> MDLMPLEKARAIEIAFDNVFHNTKIPD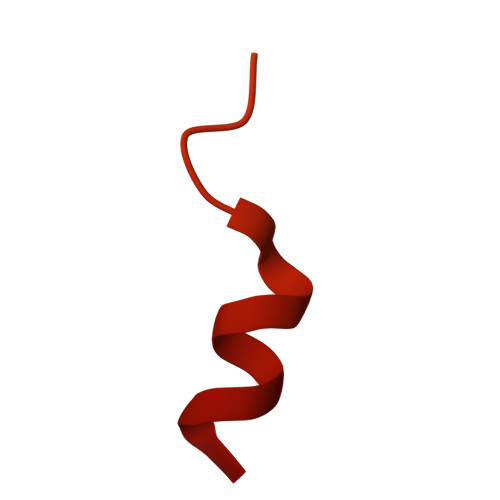NLQQFDAILKRLERRRFIPTENQKPRVYETELLVLRFREFGVKDNHNHPINLHSLRSKSLIRAQGKKLDLHNRVFLRRNVRAVKM PqsBC, a key enzyme in the biosynthesis of the quorum-sensing signal molecules HHQ and PQS and a member of the β-ketoacyl-ACP-synthase III family of condensing enzymes, has unique features of a heterodimeric subunit composition and the lack of the canonical active-site asparagine. Alternatively, it can be channeled into HHQ biosynthesis by the activity of PqsBC, which catalyzes the condensation of 2-ABA and octanoyl-CoA to form HHQ. FabH-like enzymes are usually homodimers in solution; however, the PqsBC crystal structure we report here reveals that PqsB and PqsC form a novel heterodimer. PqsC lacks the conserved asparagine, and PqsB lacks all three conserved residues of the FabH catalytic triad, raising the question of how PqsBC mediates the condensation reaction.

PqsBCC129A crystallized in space group P212121 and the structure was determined to 2 Å resolution with the final model refined to crystallographic R-factors of Rwork = 0.190 and Rfree = 0.237. The crystallographic asymmetric unit contains four copies of PqsB and four copies of PqsC. An analysis of the interfaces reveals a large ∼2,238 Å2 surface area buried by interactions formed between the PqsB and PqsC subunits as shown in Fig. 2A. The structure is thus referred to as the PqsBCC129A heterodimer. This large interface between PqsB and PqsC is observed to be almost identical in the four copies observed in the asymmetric unit (values of buried surface area are 2,277, 2,240, 2,223, and 2,212 Å2 averaged to 2,238 Å2), and the heterodimers superimpose onto each other well with an average root mean square deviation of 0.243 Å (8,182 atoms). The fold of PqsC and PqsB is closely related to the FabH enzymes and PqsD with two subdomains each composed of a four-stranded β-sheet surrounded by α-helices. Substantial differences occur in the C-terminal subdomains with PqsB having a shorter sequence (124 amino acids) with only two α-helices and PqsC (160 amino acids) having four α-helices. The active-site residues His-269 and the mutated Ala-129 (replacing Cys-129) are clearly defined in the electron density. In a noticeable difference with other members of the FabH enzyme family, an asparagine amino acid does not form a catalytic triad with His-269 and Cys-129, and in its place a valine (Val-299) is present (Fig. 3B shows the superposition of PqsC with the PqsD catalytic triad). Pro-242 breaks the helix α5 in PqsC and directs an alternate path for the polypeptide compared with FabH/PqsD forming an irregular loop structure, termed loop A, which effectively opens up the active site cleft. The shortened PqsC helix α5, a prominent difference to PqsD and FabH, widens the entry to the catalytic site and provides an extended cavity that could accommodate a bicyclic molecule such as the reaction product HHQ.

>MLIQAVGVNLPPSYVCLEGPLGGERPRAQGDEMLMQRLLPAVREALDEAAVKPEEIDLIVGLALSPDHLIENRDIMAPKIGHPLQKVLGANRAHVFDLTDSSLARALYVVDTLASDQGYRNVLVVRGESSQGLEVDSESGFALADGALALLCRPTGKAAFRRGALGGDPAQEWLPLSIPLNTDIRQVGDVKGHLNLPAQPGLPEAVRAGFTRLAGDFPQLNWVREEWFGQGRPDGRCLGPFELASQLRAAQRDRLDELLLISFDPFGMVVEGVTLELAGEAHA[4x];>[4x]SAGHKVKLAAITCELPARSYENDDPVFAAVPDLSESWWQFWGVNRRGYFDPRNGENEFSLVVRAAERLLRSSDTAPDSVDMLICSASSPIMTDAGDVLPDLRGRLYPRMANVLSKQLGLSRALPLDSQMEAASFLLNLRLAASMIRQGKAEKVLVVCSEYISNLLDFTSRTSTLFADGCAVALLTRGDDDSCDLLASAEHSDATFYEVATGRWRLPENPTGEAKPRLYFSLFSDGQNKMASFVPTNVPIAMRRALEKAGLGSDDIDYFVFHQPAPFLVKAWAEGIGARPEQYQLTMGDTGVMISVSIPYTLMTGLREGKIRPGDRIVMAGAATGWGFAAQVWQLGEVLVC> MGSSHHHHHHHHENLYFQSAGTESLDL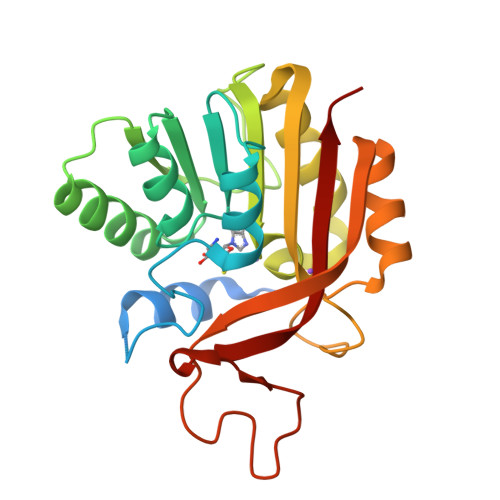EFESAYRGESVAFGEGVRPPWSIGEPQPELAALIVQGKFRGDVLDVGCGEAAISLALAERGHTTVGLDLSPAAVELARHEAAKRGLANASFEVADASSFTGYDGRFDTIVDSTLFHSMPVESREGYLQSIVRAAAPGASYFVLVFDRAAIPEGPINAVTEDELRAAVSKYWIIDEIKPARLYARFPAGFAGMPALLDIREEPNGLQSIGGWLLSAHLG> AAGTAKGHNPTEFPTIYDASSAPTAANTTVGIITIGGVSQTLQDLQQFTSANGLASVNTQTIQTGSSNGDYSDDQQGQGEWDLDSQSIVGSAGGAVQQLLFYMADQSASGNTGLTQAFNQAVSDNVAKVINVSLGWCEADANADGTLQAEDRIFATAAAQGQTFSVSSGDEGVYECNNRGYPDGSTYSVSWPASSPNVIAVGGTTLYTTSAGAYSNETVWNEGLDSNGKLWATGGGYSVYESKPSWQSVVSGTPGRRLLPDISFDAAQGTGALIYNYGQLQQIGGTSLASPIFVGLWARLQSANSNSLGF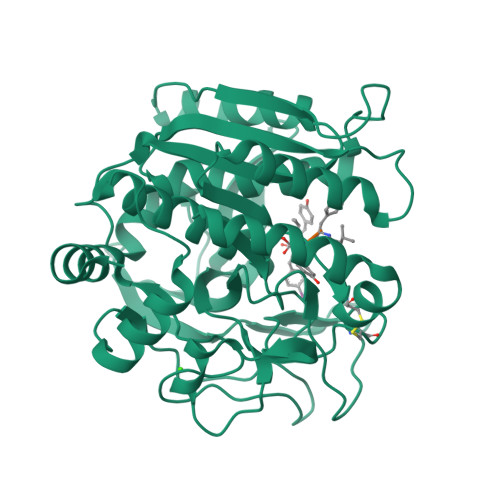PAASFYSAISSTPSLVHDVKSGNNGYGGYGYNAGTGWDYPTGWGSLDIAKLSAYIRSNGF>GSSGSSGPSQVAFEIRGTLLPGEVFAICGSCDALGNWNPQNAVALLPENDTGESMLWKATIVLSRGVSVQYRYFKGYFLEPKTIGGPCQVIVHKWETHLQPRSITPLESEIIIDDGQFGIHNGVESGP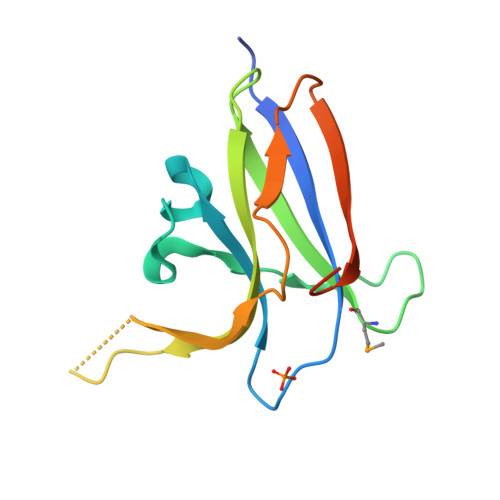SSG[6x]3-(4-bromophenyl)imidazo[2,1-b][1,3]thiazole 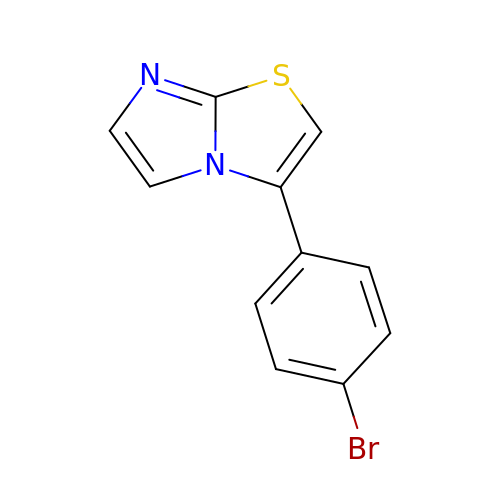| C11 H7 Br N2 S | LVDOGHLCDFUJNK-UHFFFAOYSA-N>MIALAVSGALLSSMTPAVAQPQNPDDAAIAQAEEN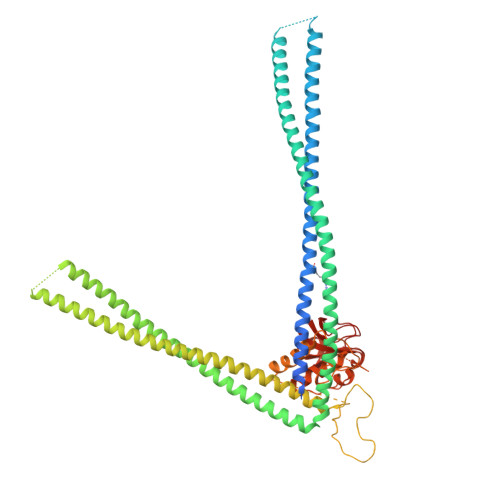VSAGDGEVARLAGSLSSTDAEINRVELEMGALREEVNKSLVDLHDAQAIAEQARQDALAAKKDLDDSQAQIEAAQERLDEISRAAYRQNGTSKGLSGISGNGNSEDALDRQTYLRTSAEKQQAAVEELDRLRTENANKESVLRQARIVAEQREAEAVEKQVQTEAAIAANSEQLNVLTNNRSTLVAQRDGAERNLAIARAQADNLQGQRAEYEEFQQAEQARIQAEAEAQAAAEEKRRADEAAAQAAAEAQEAAQQAQAAEEAQAAQAAETAQAQAAQAAETQAAQAAQAQAEANDRAAAQQRAAEAQAAAEQAQREADAQAANDAQAQALREQALTAASIAAAALIAASQSSHATTQNPYPTDEDADPTDIADIQGPTQPGTGESGDSQSNSSDNDSTGNDSTGSDSSDSDSSGNDSSEVISGDRSAQIETVIARAMSQLGVQYAWGGGNANGPTLGIRDGGVADSYGDYNKVGFDCSGLTLYAFAGVGISLPHYTGYQYQHGTKVSPSEMQRGDLIFYGPGASQHVAIYLGDGQMIEAPNSGSVVKISPVRWSGMTESVVRLI[2x]> MAEVITVKQTNMENIYECEFNDGSFRLCTRNLVPNFNVYGERLIKYEGVEYREWNAFRSKLAGAILKGLKTNPIRKGTKVLYLGAASGTTISHVSDIIELNGKAYGVEFSPRVVRELLLVAQRRPNIFPLLADAR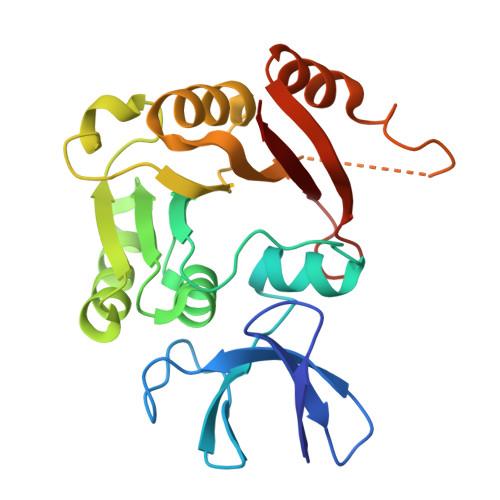FPQSYKSVVENVDVLYVDIAQPDQTDIAIYNAKFFLKVNGDMLLVIKARSIDVTKDPKEIYKTEVEKLENSNFETIQIINLDPYDKDHAIVLSKYKG> MNIRLHGLTTILSALVVLTAPTAVLAQDNLVTGELITTVNSGTPGKGGEVTFAVTRDITNWNVTSALGNNAVVRTVTLPIVPSAFMVQPDFTLKMNTDLLESAELTSTDPQTVVYRIREDAVWSDGVPITGDDFIYFWKTQNRRDCPECLINASYGHDFIETLEQDETGKVVTATFSEPFLGWQGLFMFLYPAHLAEKHGDIAESYNNFLSNEVPAWSGGPYMVESFDPGQLVTLVPNPKWYGEKGPYLDKLKFRIITDSTQQLTALENGEVDVIYPQGATQDMVEQAAGLDYLGIDFQMNPSANWYFMGLNSKAGPMSDIALRKAVLTAIDAGDLKAKTADPYLRNWPHMGSVMFLPNQAGYADRRGARGYGTGDVEKAKGILSEAGYKLSGGSLLDPSGKPVSTLRLSFPPGYPAANDMARLITGYIAPLGLKTDLLTGPNATADYLLSGNFDLHLNYFSQQVFPAVKAGQIFLRDTRQNYFGFNDPKIEEIIGKAAAASSIEESAAILSEADELAMDYAALFPIYQLPTALIYKEAILNLRDNPNQLGPAYNTAEWGLAELEHHHHHH

The EDTA transporter system is composed of a periplasmic binding protein, EppA, and a type I ABC-type importer consisting of a heterodimer of its transmembrane domain components, EppB and EppC, and a dimer of its nucleotide binding domain component, EppD. EppA binds free EDTA, but not metal–EDTA complexes, restricting the ability of Chelativorans sp. BNC1 to use only weak metal–EDTA complexes that can dissociate to free EDTA, making it imperative to determine the biophysical mechanism of EppA’s binding specificity before any improvements to its binding capabilities can be engineered. Based on its three-domain, bilobate structure, the β2β1β3βnβ4 configuration of the core β-sheet of Domain III, and the two-β-strand hinge, EppA is a Class II Cluster C periplasmic binding protein. In summary, EppA’s affinity for EDTA, EDDA, and EGTA, and its putative affinity for other APC chelators via molecular docking, suggests that it is a general binding protein for aminopolycarboxylates.

EppA crystallized without its ligand EDTA in the tetragonal space group P43212 with one molecule in the asymmetric unit. For both structures, all but the first four N-terminal residues (Gln27 through Leu30) of the mature protein (Gln27 through Glu563) were visible, and the C-terminal His-tag from pET30a(+) was visible through its first three His residues. Based on the relatively weak (e.g., no large, hydrophobic intermolecular interfaces) crystallographic and non-crystallographic protein–protein interactions in both the P43212 and P212121 crystal lattices, EppA is monomeric, which we confirmed by calculating a molecular mass of 63 kDa for the single chromatographic peak observed by analytical size-exclusion chromatography. The tertiary structure of EppA was bilobate and composed of three domains, denoted here by convention used for periplasmic binding proteins as Domains I, II, and III. Through the comparison to other Class II Cluster C PBPs and the support by molecular docking of EDTA (Section 2.3), the interface of Domains I and III established the putative ligand-binding cleft, with one end of the cleft capped by Domain II. In its observed state, this binding cleft had a volume of 688 Å3 and was solvent accessible, as shown by the presence of 35 water molecules occupying the extended binding cleft. Highlighting the counterbalancing charges, electron densities for two sulfate ions were clearly observed to be bound electrostatically in the ligand-binding cleft by Arg56 (water-mediated), Arg74, Lys470, and Arg480. Of the four cationic residues identified by molecular docking, Arg480 was the only residue situated outside of binding cleft within a short loop (Arg477 through Gln481). The loop had two conformers: Conformer A had a refined occupancy of 60% and was held in place outside of the binding clef by Asp447, and Conformer B had a refined occupancy of 40% and was oriented toward the binding cleft.The 2-deoxy-D-ribose-5-phosphate aldolase (DERA) is an enzyme involved in nucleotide catabolism. The enzyme catalyzes the formation of C-C bonds between an aldehyde as an electrophile and acetaldehyde as a nucleophile in a highly stereoselective manner. The structures display a canonical TIM barrel fold built up of eight β-α repeats in a toroidal arrangement, with an additional N-terminal helix (α0) directly adjacent to the C-terminal helix α8 (vide infra). Furthermore, all DERAs investigated in this study form constitutive dimers.

The X-ray structures of both psychrophilic DERAs were determined with resolutions of 2.1 Å for C. psychrerythraea and 1.8 Å for S. halifaxensis. We note that the relative orientations of protomers as well as the characteristics of the dimer interface for both psychrophilic DERAs closely resemble the situation in the mesophilic (E. coli) enzyme. Comparing the substrate binding pockets of the new structures with DERAEC, no amino acid exchanges or significant conformational differences were found within a radius of 5 Å about the natural substrate (as represented by the covalent intermediate included in PDBID 1JCL12). DERAs from psychrophilic species had a similar thermostability and were around 20 K less stable than DERAEC. In contrast, helices 5 and, particularly, 6 and 7 show markedly reduced strengths of rigid contacts in the psychrophilic enzymes. The relative B-factor distribution of the backbone atoms reveals a tendency towards increased flexibility in helices 0, 6, and 7 of the psychrophilic DERAs, compared to DERAEC. Hence, our X-ray structures provide independent clues in favor of the hypothesis that adaption to low temperatures in psychrophilic DERAs involves a more flexible environment of the substrate binding pocket. While in DERASH and DERAEC the melting point of the oxidized form was still lower than the wt value, the exchange led to a marked increase of 8.4 K in thermostability in the case of DERACP. Further tests for the DERACP-A95Cox variant revealed a much longer half-life at 50 °C (>80 min vs. 1 min for the wt) and 86 ± 8% of the wt activity. Nevertheless, by installing a disulfide bridge in the interface of DERACP as a psychrophilic representative, the melting temperature could be increased.

>MSDIKAVAQRALSLMDLTSLTNTETDQEIIDLCRQAKSPAGETAAICIFPRFIPVAKKALKAQQTPHIKIATVTNFPQGNDDLDIALAETRAAVAYGADEVDLVFPYRALIQGNETIGFDMVKVCKQACSGNAKLKVIIETGELKSEELIRKASEIAINAGADFIKTSTGKVAINATPEAAKVMLTVIKNKNTAVGFKPAGGVRNADDAAIYLDLADNILGNEWADANHFRFGASSLLISLLDTLGHKSNTKSSSNYHHHHHH[2x]The defining characteristics of type IA subfamily of topoisomerases include the formation of a 5′-phosphotyrosine bond in DNA cleavage, the requirement of divalent cations, and the selective binding of single-stranded DNA (ssDNA) during catalysis. Every bacterium has at least one type IA topoisomerase related to Escherichia coli topoisomerase I for overcoming topological barriers that require ssDNA strand passage. These bacterial topoisomerase I protein sequences exhibit a high degree of sequence conservation in the N-terminal domains D1–D4, where the active site for the cutting and rejoining of a single DNA strand is located. In contrast, topoisomerase I in Mycobacterium species and related species of Actinobacteria have Topo_C_Rpt type repeated units in their C-terminal region that are different from the zinc-ribbon domain. We hypothesize that while the N-terminal domains of bacterial topoisomerase I containing the DNA cleavage active site interact with the G-strand ssDNA to create a break necessary for DNA strand passage, the C-terminal domains also need to interact with the T-strand ssDNA with high affinity.

We succeeded in obtaining a new crystal structure of a catalytically active 839-residue form of M. smegmatis topoisomerase I (MsmTOP1-839t) in complex with a 25-base ssDNA, MTS2-25. The construct MsmTOP1-839t includes the N-terminal domains (D1–D4) and three of four predicted C-terminal domains. In addition to the N-terminal toroidal assembly (D1–D4 domains) and the first C-terminal domain (D5) that have been characterized in MtbTOP1-704t structures, the second and the third C-terminal domain (D6 and D7) have also been resolved. Within the structure, the 5′-end regions of the two MTS2-25 oligonucleotides in opposite polarity form a 12-base-pair dsDNA containing six non-Watson–Crick base pairings and mismatches. In the dimer-like MsmTOP1-839t/MTS2-25 assembly, the C-terminal D6 and D7 domains of MsmTOP1-839t from one MsmTOP1-839t/MTS2-25 complex binds to the very 3′-end of MTS2-25 (5′-TTGACTT-3′) from another MsmTOP1-839t/MTS2-25 complex, and vice versa. In this pre-transition state, the active site tyrosine is in position to attack the scissile phosphate that is four nucleotides downstream of a cytosine recognized in the –4 position by a set of conserved residues. In the MsmTOP1-839t monomer A structure, the C-terminal D6 and D7 bind a ssDNA segment in a 3′ to 5′ direction. Each domain interacts with two consecutive nucleotides, primarily through two parallel π-π stackings. We do not observe here any interactions of the arginine residue on the β-turn (R724 of D6 and R805 of D7) to form salt bridges to phosphate groups of ssDNA or contribute a hydrogen bond.

>[2x]SNAMAGGDRGSGGTGNVRRLVIVESPTKARKIAGYLGSNYVVESSRGHIRDLPRNAADVPAKFKSEPWARLGVNVDQNFEPLYIVSPEKKSTVTELKGLLKDVDELYLATDGDREGEAIAWHLLETLKPRVPVKRMVFHEITEPAIRNAAENPRDLDIALVDAQETRRILDRLYGYEVSPVLWKKVAPKLSAGRVQSVATRIIVQRERERMAFHSASYWDVTAELDASVSDPSASPPKFTAKLNTVDGRRVATGRDFDSLGQLKRPDEVLVLDEASAGALASGLRGAQLAVTSVEQKPYTRRPYAPFMTSTLQQEAARKLRFSSERTMSIAQRLYENGYITYMRTDSTTLSESAINAARTQARQLYGEEYVHPSPRQYTRKVKNAQEAHEAIRPAGDVFQTPGQLHSALDTDEFRLYELIWQRTVASQMADARGTTLSLRIGGSASSGEQVVFNASGRTITFPGFLKAYVESIDELAGGESDDAESRLPNLTQGQRVDAADLSADGHQTSPPARYTEASLIKALEELGIGRPSTYSSIIKTIQDRGYVQKKGSALVPSWVAFAVVGLLEQHFGRLVDYDFTAAMEDELDEIANGQEQRTNWLNNFYFGGEHGVEGSIARAGGLKQLVGGNLEGIDAREVNSIKVFDDSEGRPVYVRVGRNGPYLERMVDDPDNPGEQKPQRANLKEDLTPDELTPELAEKLFATPQEGRSLGIDPETGHEIVAKDGRFGPYVTEVLPEPEDGGDDGTAGTPAKKGKKPTGPKPRTGSLFRSMDLETVTLEDALKLLSLPRVVGVDPTTNEEITAQNGRYGPYLKRGTDSRSLATEDQIFTITLDEALKIYAE>[2x]MRSRRVDVMDVMNRLILAMDLMNRDDALRVTGEVREYIDTVKIGYPLVLSEGMDIIAEFRKRFGCRIIADFKVADIPETNEKICRATFKAGADAIIVHGFPGADSVRACLNVAEEMG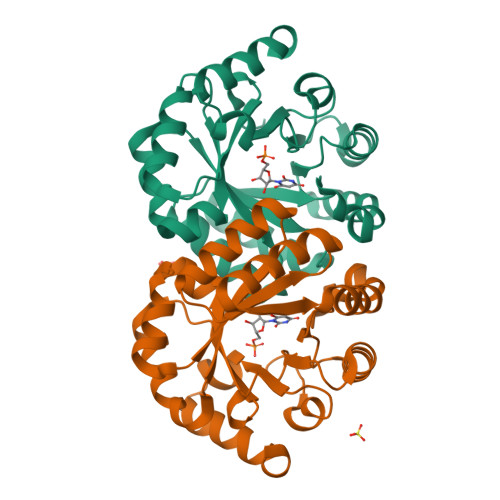REVFLLTEMSHPGAEMFIQGAADEIARMGVDLGVKNYVGPSTRPERLSRLREIIGQDSFLISPGVGAAGGDPGETLRFADAIIVGRSIYLADNPAAAAAGIIESIKDLLNP>[2x]GSASTVKGSVDLEKLAFGLTKLNEDDLVGVVQMVTDNKTPEMNVTN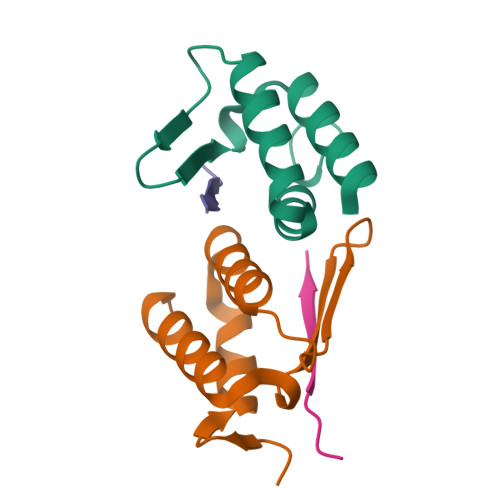NVEEGEFIIDLYSLPEGLLKSLWDYVKKNT;>SRSFMVKIRTKN[2x]>[4x]SAVKAARYGKDNVRVYKVHKDEKTGVQTVYEMTVCVLLEGEIETSYTKADNSVIVATDSIKNTIY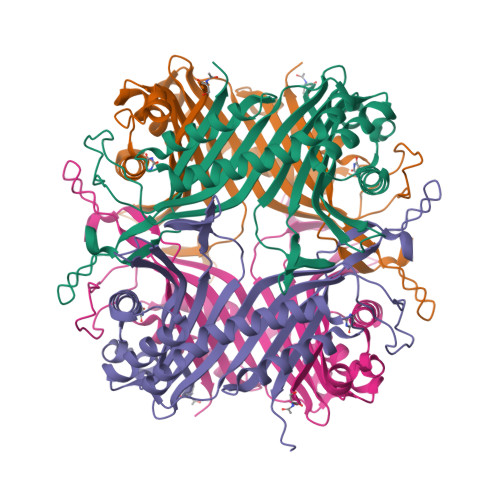ITAKQNPVTPPELFGSILGTHFIEKYNHIHAAHVNIVCHRWTRMDIDGKPHPHSFIRDSEEKRNVQVDVVEGKGIDIKSSLSGLTVLKSTNSQFWGFLRDEYTTLKETWDRILSTDVDATWQWKNFSGLQEVRSHVPKFDATWATAREVTLKTFAEDNSASVQATMYKMAEQILARQQLIETVEYSLPNKHYFEIDLSWHKGLQNTGKNAEVFAPQSDPNGLIKCTVGRSSLKSKL> MQQGQMAGGRAITVFSPDGRLFQVEYAREAVKKGSTALGMKFANGVLLISDKKVRSRLIEQNSIEKIQLIDDYVAAVTSGLVADARVLVDFARISAQQEKVTYGSLVNIENLVKRVADQMQQYTQYGGVRPYGVSLIFAGIDQIGPRLFDCDPAGTINEYK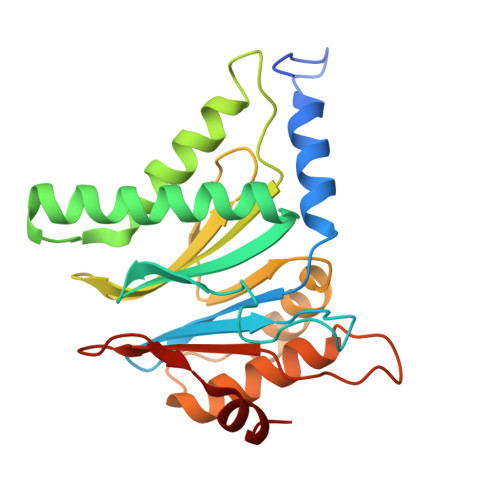ATAIGSGKDAVVSFLEREYKENLPEKEAVTLGIKALKSSLEEGEELKAPEIASITVGNKYRIYDQEEVKKFL> AGDMYIVNPDDLQLTFTMEFEVTVTRDGFHKRTISVDNGRPVVVWDGGDKDPKICKICPAVNSINTENIFLDIQKMRLNNLLAQGLWDIQRICVRYVCLFLGFDVVCDVYHTTDRVRAAYTRQTGKIDIQGSGTFSTSDAKGIGTYM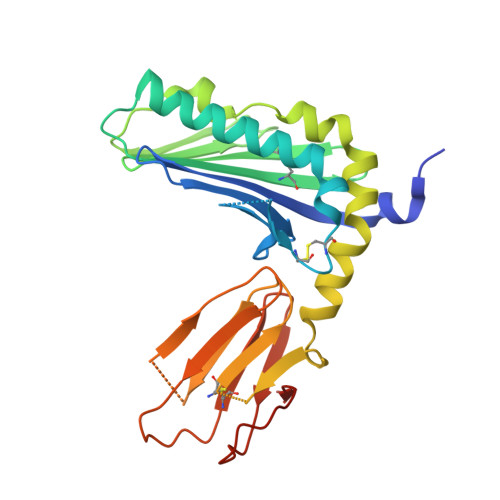IESNVREIKNKWRPTVQKLKQLGYMNETEVEFWYNTTGLTTCVVTSRSNVPFTVELSLNTNSSAIVTEESTVDCQTVTVKAPGSHAQRCYVTSSLGWKGVVTPPSQYRTKRAPVNIHHHHHH RCD1 is the founding member of a plant‐specific protein family characterized by a central domain with sequence similarity to the catalytic domain of Poly‐(ADP‐ribose)‐polymerases (PARPs) (Lamb et al., 2012). In addition to the central PARP domain, RCD1 and its paralogue SIMILAR TO RCD ONE1 (SRO1) have an N‐terminal WWE domain and a C‐terminal RST domain. RCD1 and sequence‐related proteins localize to the plant cell nucleus and bind several transcription factors via their RST domains, possibly explaining why loss of RCD1 function affects plant development and several stress signaling pathways (Katiyar‐Agarwal et al., 2006; Jaspers et al., 2009; You et al., 2014). In contrast to canonical PARPs that covalently modify target proteins by ADP‐ribosylation, Arabidopsis RCD1 does not show PARP activity in vitro when expressed as a GST fusion (Jaspers et al., 2010).

Our crystal structure of the RCD1 PARP domain provides first insights into plant PARP domains, and we identified several molecular differences between RCD1's PARP domain and the catalytic domain of mammalian PARPs. The RCD1 PARP domain adopts a fold that is overall similar to mammalian PARP domains. However, the RCD1 PARP domain structure confirmed that the amino acid triad H‐Y‐E, constituting the active site of mammalian and plant PARPs, is not conserved in RCD1 (Kleine et al., 2008; Jaspers et al., 2010). Nonconservation of the His and Tyr residues critical for NAD+ binding in canonical ADP‐ribosyl‐transferases suggests that the RCD1 PARP domain does not bind NAD+ and therefore is likely to lack canonical PARP activity. Consistent with this inference, the RCD1 PARP domain is not stabilized by 6(5H)‐phenanthridinone, an inhibitor of mammalian PARPs (Wahlberg et al., 2012), at elevated temperatures. Conceivably, the cleft of RCD1 that corresponds to the catalytic center of active PARPs has evolved to bind other small compounds. To test whether this region of the protein is required for the biological function of RCD1, we designed three RCD1 mutant variants with single amino acid exchanges in the cleft region. However, an independent transgenic line (A) expressing the same construct fully complemented both rcd1‐1 phenotypes, suggesting that differences in expression levels might account for partial complementation in line B. Overall, our results suggest that the integrity of the presumed NAD+ binding cleft is not essential for RCD1's functions in plant development and signal transduction under oxidative stress conditions. Nonconservation of the H‐Y‐E triad and our finding that RCD1 retains its biological function when amino acids within the presumed active site are mutated suggest that the protein does not have PARP activity. Given that the N‐ and C‐terminal domains of RCD1 mediate protein–protein interactions, the PARP domain of RCD1 might act as a scaffold bridging and/or coordinating the action of the terminal protein interaction domains.

>GPGSEVLDKDAVKKMFAVGTASLGHVPVLDVGRFSSEIAEARLALFQKQVEITKKHRGDANVRYAWLPAKREVLSAVMMQGLGVGGAFIRKSIYGVGIHLTAADCPYFSARYCDVDENGVRYMVLCRVIMGNMELLRGDKAQFFSGGEEYDNGVDDIESPKNYIVWNINMNTHIFPEFVVRFKLSNLPNAEGNL[8x]> PY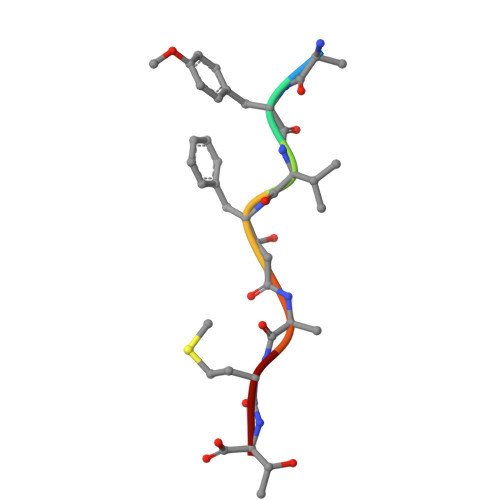VFAMT(2~{S})-2-[[(3~{S},4~{R},5~{R})-3,4,5,6-tetrakis(oxidanyl)-2-oxidanylidene-hexyl]amino]pentanedioic acid | C11 H19 N O9 | 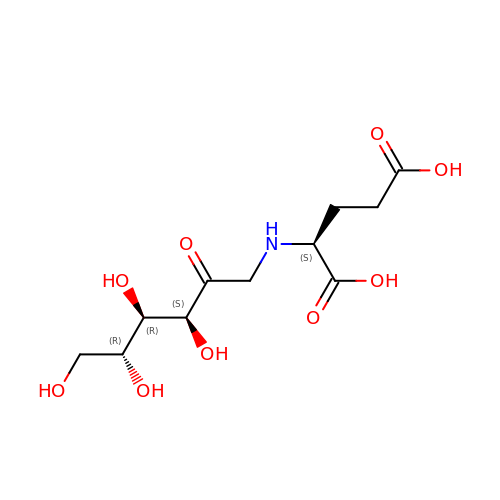PUFNBARRTADWAC-AJGMQJJTSA-N2-amino-8-(trans-4-methoxycyclohexyl)-4-methyl-6-(1H-pyrazol-3-yl)pyrido[2,3-d]pyrimidin-7(8H)-one 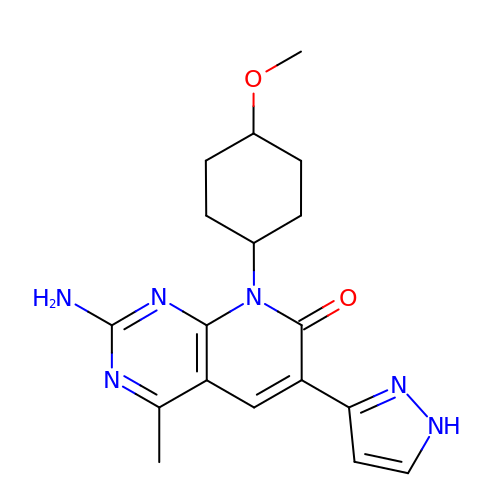| C18 H22 N6 O2 | UDXSDTPXGCELRI-HAQNSBGRSA-N>HMLEENIQEKIAFIFNNLSQSNMTQKVEELKETVKEEFMPWVSQYLVMKRVSIEPNFHSLYSNFLDTLKNPEFNKMVLNETYRNIKVLLTSDKAAANFSDRSLLKNLGHWLGMITLAKNKPILHTDLDVKSLLLEAYVKGQQELLYVVPFVAKVLESSIRSVVFRPPNPWTMAIMNVLAELHQEHDLKLNLKFEIEVLCKNLALDINELKPGNLLKDKDRLKNLDEQLS[3x];>[3x]MPAATVDHSQRICEVWACNLDEEMKKIRQVIRKYNYVAMDTEFPGVVARPIGEFRSNADYQYQLLRCNVDLLKIIQLGLTFMNEQGEYPPGTSTWQFNFKFNLTEDMYAQDSIELLTTSGIQFKKHEEEGIETQYFAELLMTSGVVLCEGVKWLSFHSGYDFGYLIKILTNSNLPEEELDFFEILRLFFPVIYDVKYLMKSCKNLKGGLQEVAEQLELERIGPQHQAGSDSLLTGMAFFKMREMFFED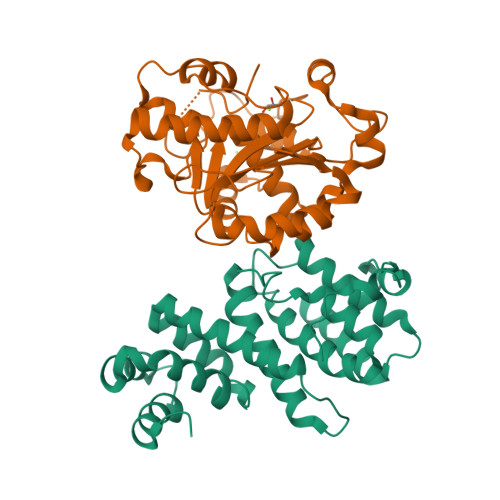HIDDAKYCGHLYGLGSGSSYVQNGTGNAYEEEANKQS>[5x]MFSGIKGPNPSDLKGPELRILIVHARWNLQAIEPLVKGAVETMIEKHDVKLENIDIESVPGSYELPQGIRASIARNTYDAVIGIGVLIKGSTMHFEYIS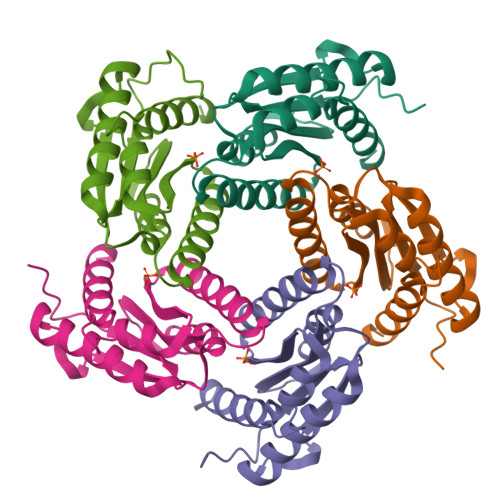EAVVHGLMRVGLDSGVPVIFGLLTVLNEEQALYRAGLNGGHNHGNDWGSAAVEMGLKALY>[3x]MKKIYFMLAIAGIFAGCVPSANSATKNSSANSTAPSQDVIVQKVDKDDVRDIIREEKMLAPDASETELSFTAVGEGIAPMNTVSTAQALALAKRAAITDAYRQLASKLYGVKVNGKDTVKDAMLRSSTITAQVNGLIKNASIIDENFNQGLYRVNLELKIDADKWKELFAY;>MKKILIICMLFTLSFGIERPKFEDFLAGYERNKASMLNYEGMPAFALSENLLAVLKQPNTKLNKYVKYDPFLNLYLVRTDFSLIPTPMGDEEKLTRNDWVGIWDPNKPYIGHIKYLAQNIDEKDQLDFNSKIGLLGTPCCEMMGIALNNSSFIGNRYLKHFMKYNDVYWGDIGVDFVVRENKIYVNNVRKNPQFLINDQVISVDGLPANDLRKLNEKILFADRGSTLYFQVLRDNMDLNISTEVFAKDLSKFNLPDSKPKPKITNFTSNLGLTVNTSLVVTKIDPKSKASNAGFMVGDKILRVNNIILNNFKELQNILSAGNDFSILIERKSTKLPLSNFNNELGGNANSGGDGKFQFFIRLTK[7x];> MRILFLILLSFLNAFAFELVLNTGRENNQAFAVLHASNDLEFTCQKFITEAKVHFECDIVGMVDNKLKDQSFSAFDLKFIQEAQKIKMIILPKIQARMFDTSQNIYIDKELSSSSSHKSKAFTFIFTPELAPIKDYDGLDFNINFPHESLPYVGALDLNSDPVVIPQSADINTYLRIKKEYDKANYNQVVIDAQNAINRYRGSIFTSEFILYKLRAQNKLYTQDPSMRDQQILEKMIDDAKNWTRTFTSDKNFSEVLHIMLRTYIALAQRADVEYTMSILDNEQPNNYFTQLSKLDYADYIYNLNEKEKAVNIYENTYFNTKNLDLAARAAMSLAKNLLSNEQVNKAIEYINTILKANPEYFGKDIPRSLELAKLFNQKGQFDISASIYEDAFAKMSKLDPSYEETLKDLALVLSHANRSSDAKKYLDLYMDDYLDGKYLDEIKKASDEVFFALGDNNASFLHQRYTDLMKQYANKDENIANKALDEDVALYYKEGNFSAILAYKDLIESKKIPNATQFLEKAAINDLKNAIKADNCINAANIFMRFSAYDIGQKIENKKQMLACLIRTSNVEQALDYIDKNYNEDSIFYGLQKASILFDNKQYPQVIKISKDIANSRILKSDDENFKAYYLQFLSLLRLNDYNQAIKILQILESFPMNFSMVEAYDALLSYANDHNMQTTILTYAPKAIDYQNFKGINLFSPNLEFIYLDALTKINKNEESLAVLTDLLKLKLSDEDRARALYIQALTYERMQNIQAEKESLKQCLEIKSASNWQNLCKSKNQILNQ;> MAEQEDIILEKPEDGLNQPRLDESLEGFKGQEGQAPEDEEFASLPEELPQENSESGFKFTRESAPEDVSTFEEVESQEPTPWYKDRKFMSLVGLSLGIICILVFTLFYLTFSEGKIKPDIIASKPLEQPVVMPDESYKYNDMQRIDGMIQKANALYLKGEVEQALKVYEQVAVYNESLSNYNLGVSQMNENKFQEAFESFKKAIANGENQSVAAINAAVCALKLNDKEKFRYYIDLAQVYLPKEGKSKLYDYYLSLINYYKGYYPEALQMLQRTDMEPYSDVAKYLSAKIYAKMDFDSKAIQQLNSQGNFESSLSLGLLYARIGEYAKAKVALSTAMKIERDFNQSLAALTLVDIKTGNYQDMLARLQNSYDNDKDRYKILDAYKIQVRLNKDLFNIAVAQNSFSKDLLKKQKDQFDLLFYFAPYQVFDSKQAALYIKKANVTDFVDDSADAGVYLNTSKALSSTNVKIANIINYALNQKLRLANQEFQKLIKDYPEHSILHYNLALTYAQMQNYELAYKHFSSSYHLNPKNYLAGAFAMFCAKLIDIDTTKLYNEILDNIAADSNFKANMQKSMLFLVNNNYISMLPYLDETKKDTPLSLIFEAIVAKNNNLNNQVDVKIAKLRSELPEDILANILYFNSLNSNLNIKEYAQNAQIHFKNLKLDYRSVFGGPNIAREFYVNLMHIAGLLNLERQKIKELINVSGAKDEGILQTLAYLDIFAQQYEEAYALYNSLIDDYGAKDTKTLFLAAVAAIGANNPNSAIALLQLSKLTDKNNKESKAALGMLYQEVKNYEAAISQYKTLPNNFKSEFFTFDINNN;>MAKKHKCPECPAGEKWAVPYADFLSLLLALFIALWAISKTNPAKVEALKTEFVKIFDYTSTQTVKEESKTQEKYKGAAKEESDELKSLKQMTMTQQETIKRLQAALDQSDNQVALNLPSKVEFERGSAQIVSADIQDYLKRMAELTTYLPPQAKIEIRGYTDNSDSIIRSYELAYQRAENVLKYFIEGGANLKNISIKSYGLNNPINGNPQALENNRVEIYFKVDTADTSTQKSVLELINKIGTKAP[2x];>MDEELENEETKKKKGGSLVIIIVILLFVLLLSIMGVIAWLISSSSSDESEVKEAPKEEAKADKPKVSAPTQRGSDFANIGPMYPLDPFTLNLLSDSGSRYVKCTIELEQNSELLKPELDKKVPVIRDIIIRTLTAKTFEEVSTQKGKERLKDELVGKINEILTDGFIKNVYFTDFVVS[4x]

The bacterial flagellar motor, which spins a helical propeller for propulsion, has undergone evolutionary diversification across bacterial species, often involving the addition of structures associated with increasing torque for motility in viscous environments. Here we developed a Campylobacter jejuni minicell system for in situ cryogenic electron microscopy imaging and single-particle analysis of its motor, one of the most complex flagellar motors known, to subnanometre resolution. The basal disk is formed of FlgP; the medial disk of PflC and PflD; and the proximal disk of PflA, PflB and FliL together with stator complex components MotA and MotB.

Given that these symmetry-mismatched regions comprise universally conserved structures (such as the P-, L-, MS- and C-rings) and the stator complexes which have already been structurally characterized, we focused on C. jejuni’s relatively recently evolved 17-fold symmetric periplasmic scaffold structures. Bending the arc of these oligomers demonstrated that 17 trimeric repeats, that is, 51 protomers, fit into the 51 periodic densities of the innermost ring of the basal disk, with a map-model FSC of 9.9 Å at FSC = 0.5. FlgP, however, features an additional C-terminal helix and long β-hairpin insert between the SHS2 α-helix and the second SHS2 β-strand. This β-hairpin insert extends 35 Å at a ~42° angle to the vertical axis and is the basis of the continuous β-sheet in the inner face of each FlgP concentric ring. PflCC docks to the underside of the first ring of FlgP, while PflCN forms the inner band of the medial disk; a density corresponding to the linker bridges adjacent PflC protomers, indicating that the PflCC domain of one chain assembles with the PflCN domain of another in a daisy chain of domain-swapped protomers. The remainder of the medial disk is a lattice of α-helices that we could interpret with 17 asymmetric units of 6 additional PflCN protomers in a lattice. We inspected the peripheral part of the medial disk adjacent to PflC4 which disappeared when we deleted pflD, and found that a model of PflD was consistent with this density, despite the lower resolution of this area of our map yielding only a modest mean main chain correlation coefficient of 0.63. We flexibly fitted these structures into our map, resulting in a structure in which 17 radial spokes of PflA position a continuous rim of 17 PflBs. PflAB heterodimerized even at nanomolar concentrations, while deleting the linker and β-sandwich domain of PflA (residues 16–168) abolished dimer formation.>[8x]MGSSHHHHHHSSGRENLYFQGMLLPETRNLLDLMDAATRGGRPRLETLPHAVGRKAVDKMSEDGEADPPEVAEVANGGFAGPASEIRFRRYRPLGEAAGLLPTLIYYHGGGFVIGNIETHDSTCRRLANKSRCQVISIDYRLAPEHPFPAPIDDGIAAFRHIRDNAESFGADAARLAVGGDAAGGAMAAVVCQACRDAGETGPAFQMLIYPATDSSR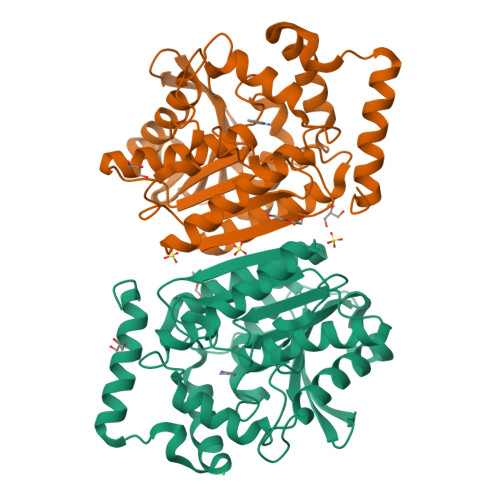ESASRVAFAEGYFLSKALMDWFWEAYVPEDTDLTDLRLSPLLATDFTGLPPAFVLTAGYDPLRDEGRAYADRLIEAGIKTTYVNYPGTIHGFFSLTRFLSQGLKANDEAAAVMGAHFGT> GTAPKVLFTGVVDARGERAVLALGGSLAGSAAEASHLVTDRIRRTVKFLCALGRGIPILSLDWLHQSRKAGFFLPPDEYVVTDPEQEKNFGFSLQDALSRARERRLLEGYEIYVTPGVQPPPPQMGEIISCCGGTYLPSMPRSYKPQRVVITCPQDFPHCSIPLRVGLPLLSPE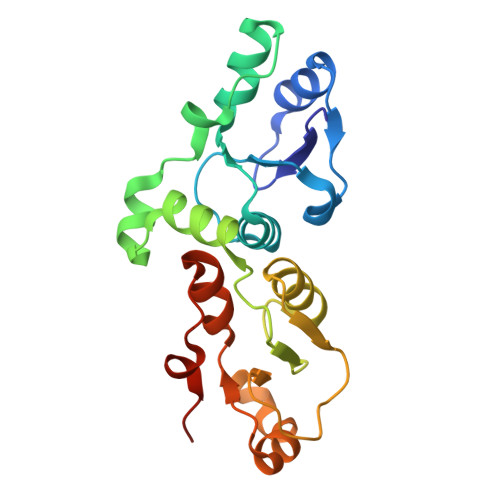FLLDGVLKQEAKPEAFVLSPLEMSST> RSIIGGKHGDRDVRILYQVGDSEEDLPVCAPNAVCSKIDLYETPWIERQCRCPDG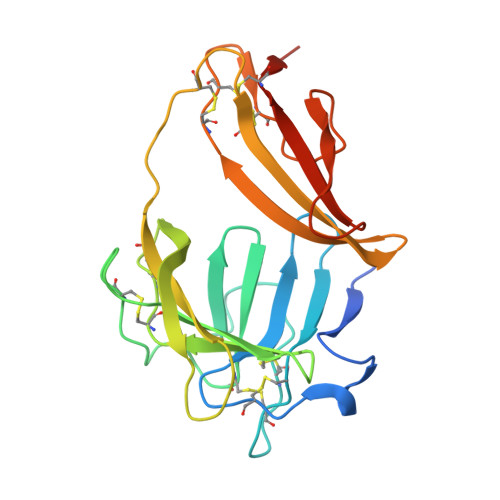RTCPSSLGVEDGHTIADKTRHYKMCQPVHKLPVCKHFRDYTWTLTTAAELNVTEQIVHCRCPRNSVTYLTKREPIGNDSPGYRYLFACSPLTRLRCQRKQPCKLFTVRKRQEFLDEVNINSLCQCPKGHRCPSHHTQSGVIAGESFLEDNIQTYSGYCMANDHHHHHH>MNTTPVHALTDIDGGIAVDPAPRLAGPPVFGGPGNDAFDLAPVRSTGREMLRFDFPGVSIGAAHYEEGPTGATVIHIPAGAR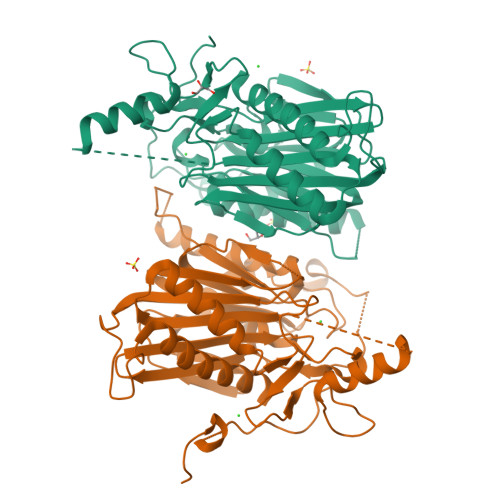TAVDARGGAVGLSGGYDFNHAICLAGGAGYGLEAGAGVSDALLERLEHRTGFAELQLVSSAVIYDFSARSTAVYPDKALGRAALEFAVPGEFPQGRAGAGMSASAGKVDWDRTEITGQGAAFRRLGDVRILAVVVPNPVGVIVDRAGTVVRGNYDAQTGVRRHPVFDYQEAFAEQVPPVTEAGNTTISAIVTNVRMSPVELNQFAKQVHSSMHRGIQPFHTDMDGDTLFAVTTDEIDLPTTPGSSRGRLSVNATALGAIASEVMWDAVLEAGK[2x]>[6x]GPGSMARNKIALIGSGMIGGTLAHLAGLKELGDVVLFDIAEGTPQGKGLDIAESSPVDGFDAKFTGANDYAAIEGADVVIVTAGVPRKPGMSRDDLLGINLKVMEQVGAGIKKYAPEAFVICITNPLDAMVWALQKFSGLPAHKVVGMAGVLDSARFRYFLSEEFNVSVEDVTVFVLGGHGDSMVPLARYSTVAGIPLPDLVKMGWTSQDKL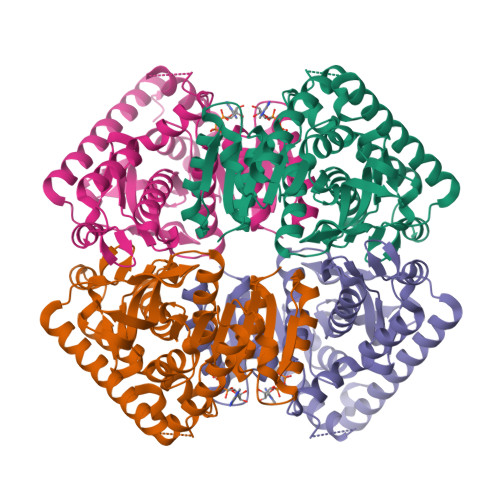DKIIQRTRDGGAEIVGLLKTGSAFYAPAASAIQMAESYLKDKKRVLPVAAQLSGQYGVKDMYVGVPTVIGANGVERIIEIDLDKDEKAQFDKSVASVAGLCEACIGIAPSLK> CVFCRLPAHDLSG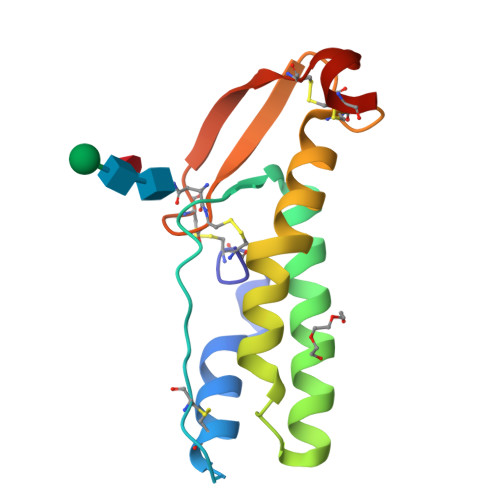RLARLCSQMEARQKECGASPDFSAFALDEVSMNKVTEKTHRVLRVMEIKEAVSSLPSYWSWLRKTKLPEYTREALCPPACRGSTTLYNCSTCKGTEVSCWPRKRCFPGS> WAEEPTFRLEFKDGVITPDRLEVPANTRFRIELVNTGSMPAEFESLELRKEKVIAAQSETVMVIRTLDPGEYPFFDDFHPGGTPAILIAK

FtrABCD is a four-component iron transporter found in several Gram-negative bacteria. Previous data confirm that FtrABCD can only utilize Fe2+ and the inner membrane permease, FtrC, from this system, like its eukaryotic homologue, Ftr1p, is predicted to utilize the free energy released during Fe2+ oxidation for the transport. Periplasmic FtrB from this system is coancestral with known copper oxidases, and the conserved D118 and H121 are predicted to bind to Cu2+, forming an active enzyme. On the other hand, we and another group predicted that periplasmic FtrB (10 kDa) is a novel cupredoxin (Cup-II) based on its common ancestry with Fet3p (a multicopper oxidase) and other single-domain cupredoxins.

We investigated the validity of this phylogenetic prediction by crystallizing recombinant wild-type apo-FtrB from Brucella abortus 2308 (see Materials and Methods section for details about making apo-proteins from as-isolated proteins) from 100 mM sodium acetate (pH 4.6), 20% (v/v) polyethylene glycol 3350, and 20–100 mM MnCl2 supplemented with 20–100 mM CuSO4 and obtained diffraction data at 1.30 Å resolution. The final refined structure (Rfree = 19.8%) at a limiting resolution of 1.30 Å was produced. For example, structural fold analysis of FtrB revealed the presence of nine β-strands, resulting in three β-sheets through H-bond interactions (Sheet1:1–2–4–7, Sheet2:3–8–9, and Sheet3:5–6). Interestingly, the electron density that can correspond to the presence of copper metal close to the D118 and H121 residues was not identified. This can be due to several reasons, such as the pH of crystallization being 4.6, where the side chain of H121 would be protonated and hinder Cu2+ binding (pKa for H121 in FtrB using ProPKA 6.5).21 Second, acetate being a competitive chelator for Cu2+ and being present in such a high concentration under the crystallization condition (100 mM acetate and 10–100 mM CuSO4). In contrast, diffraction data from wild-type FtrB crystals showed that two large peaks of unmodeled density above 5σ were found in the Fo–Fc difference map and could be modeled as two Mn2+ ions with high occupancy (Mn1 = 0.88 and Mn2 = 0.71) and low B-factors (Mn1 = 15.54 Å2 and Mn2 = 14.20 Å2). Coordination of Mn1 is mediated by side chain oxygen atoms of residues E84 and E86 (from the EXE motif), E93 (from the RKEKV motif), and D119 and two ordered waters, resulting in octahedral geometry. A second Mn2+ (Mn2) is found 5.3 Å from Mn1, near the loop connecting β-strands 5 and 8.14−16 Surprisingly, only a single coordinating ligand originates from FtrB (i.e., D119), with five oxygen atoms from ordered water molecules acting as the remaining coordinating ligands, resulting in octahedral geometry. Despite this flexibility, all FtrB conserves E86 and E93 residues, which are seen to coordinate to a Fe2+ mimic in our crystal structure, and we conclude that FtrB plays a crucial role in iron transport.> MKPASQRGSVDGLGSSLPIASMLPAVFADDDLALRFVAGLDDVLAPILNVLDCLDTYFDPALTPADFAQWLGTWVGAETDGTEAEPMLRAAVAAAARLHRVRGTLQGLSETVRLAFGVAPEITESGGATWNARPLGPF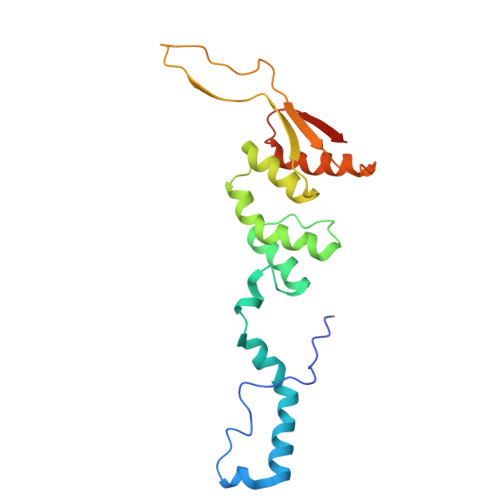PGRPRPQLHVALRLPEPRPVDVHRLDALVAAARPAHMPYTVEVTASERTPER> MGSSHHHHHHSSGLVPRGSPQPPADEQPEPRTRRRAYLWCKEFLPGAWRGLREDEFHISVIRGGLSNMLFQCSLPDTTATLGDEPRKVLLRLYGAILQMRSCNKEGSEQAQKENEFQGAEAMVLESVMFAILAERSLGPKLYGIFPQGRLEQFIPSRRLDTE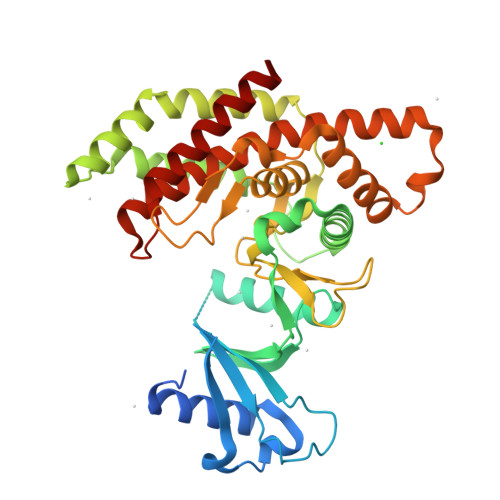ELSLPDISAEIAEKMATFHGMKMPFNKEPKWLFGTMEKYLKEVLRIKFTEESRIKKLHKLLSYNLPLELENLRSLLESTPSPVVFCHNDCQEGNILLLEGRENSEKQKLMLIDFEYSSYNYRGFDIGNHFCEWMYDYSYEKYPFFRANIRKYPTKKQQLHFISSYLPAFQNDFENLSTEEKSIIKEEMLLEVNRFALASHFLWGLWSIVQAKISSIEFGYMDYAQARFDAYFHQKRKLGV> MEYKSSPKRPYLLRSLYDWLVDNSFTPYLVVDATYL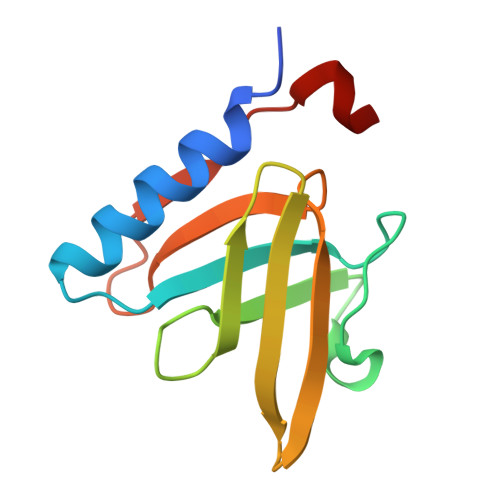GVNVPVEYVKDGQIVLNLSASATGNLQLTNDFIQFNARFKGVSRELYIPMGAALAIYARENGDGAMFEPEEIYDE> FVEMVDNLRGKSGQGYYVEMTVGSPPQTLNILVDTGSSNFAVGAAPHPFLHRYYQRQLSSTYRDLRKGVYVPYTQGKWEGELGTDLVSIPHGPNVTVRANIAAITESDKFFINGSNWEGILGLAYAEIARPDDSLEPFFDSLVKQTHVPNLFSLQLCGAGFPLNQSEVLASVGGSMIIGGIDHSLYTGSLWYTPIRREWYYEVIIVRVEINGQDLKMDCKEYN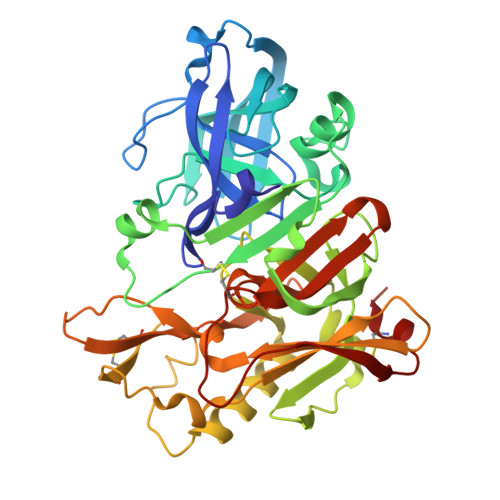YDKSIVDSGTTNLRLPKKVFEAAVKSIKAASSTEKFPDGFWLGEQLVCWQAGTTPWNIFPVISLYLMGEVTNQSFRITILPQQYLRPVEDVATSQDDCYKFAISQSSTGTVMGAVIMEGFYVVFDRARKRIGFAVSACHVHDEFRTAAVEGPFVTLDMEDCGYNI> MRSRRVDVMDVMNRLILAMDLMNRDDALRVTGEVREYIDTVKIGYPLVLSEGMDIIAEFRKRFGCRIIADFKVADIPETNEKICRATFKAGADAIIVHGFPGADSVRACLNVAEEMGREVFLLTEMSHPGAEMFIQGAADEIARMGVDLGVKNYVGPSTRPERLSRLREIIGQDSFL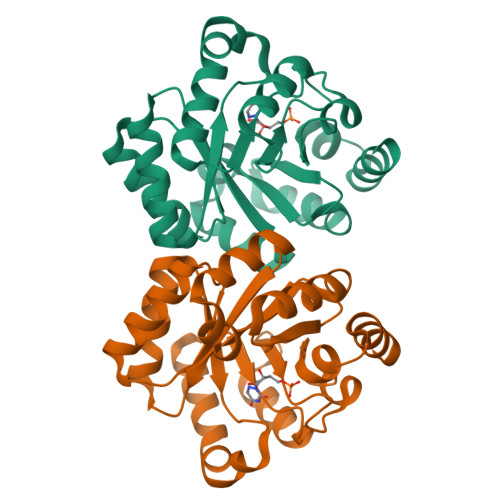ISPGVGAAGGDPGETLRFADAIIVGRSIYLADNPAAAAAGIIESIKDLLIPEDPAANKARKEAELAAATA> MAVLGLQGVRGGVGTTTITAALAWSLQMLGENVLVVDACPDNLLRLSFNVDFTHRQGWARAMLDGQDWRDAGLRYTSQLDL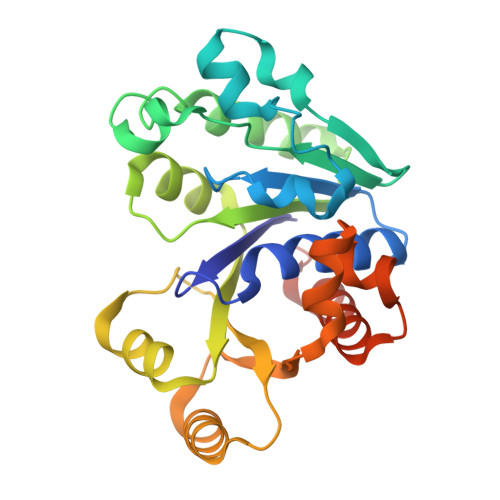LPFGQLSIEEQENPQHWQTRLSDICSGLQQLKASGRYQWILIDLPRDASQITHQLLSLCDHSLAIVNVDANCHIRLHQQALPDGAHILINNFRIGSQVQDDIYQLWLQSQRRLLPMLIHRDEAMAECLAAKQPVGEYRSDALAAEEILTLANWCLLNYSGLKTPVGSKS> MESHVKYLDELILAIKDLNSGVDSKVQIKKVPTDPSSSQEYAKSLKILNTLIRNLKDQRRNNIMKNDTIFSKTVSALALLLEYNPFLLVMKDSNGNFEIQRLIDDFLNISVLNYDNYHRIWFMRRKLGSWCKACVEFYGKPAKFQLTAHFENTMNLYEQALTEVLLGKTELLKFYDTLKGLYILLYWFTSEYSTFGNSIAFLDSSLGFTKFDFNFQRLIRIVLYVFDSCELAALEYAEIQLKYISLVVDY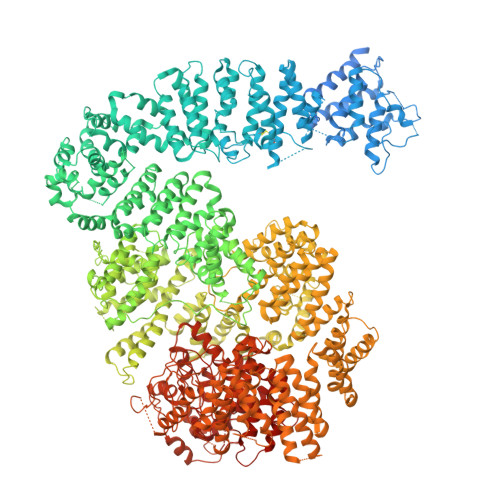VCNRTISTALDAPALVCCEQLKFVLTTMHHFLDNKYGLLDNDPTMAKGILRLYSLCISNDFSKCFVDHFPIDQWADFSQSEHFPFTQLTNKALSIVYFDLKRRSLPVEALKYDNKFNIWVYQSEPDSSLKNVTSPFDDRYKQLEKLRLLVLKKFNKTERGTLLKYRVNQLSPGFFQRAGNDFKLILNEASVSIQTCFKTNNITRLTSWTVILGRLACLESEKFSGTLPNSTKDMDNWYVCHLCDIEKTGNPFVRINPNRPEAAGKSEIFRILHSNFLSHPNIDEFSESLLSGILFSLHRIFSHFQPPKLTDGNGQINKSFKLVQKCFMNSNRYLRLLSTRIIPLFNISDSHNSEDEHTATLIKFLQSQKLPVVKENLVIAWTQLTLTTSNDVFDTLLLKLIDIFNSDDYSLRIMMTLQIKNMAKILKKTPYQLLSPILPVLLRQLGKNLVERKVGFQNLIELLGYSSKTILDIFQRYIIPYAIIQYKSDVLSEIAKIMCDGDTSLINQMKVNLLKKNSRQIFAVALVKHGLFSLDILETLFLNRAPTFDKGYITAYLPDYKTLAEITKLYKNSVTKDASDSENANMILCSLRFLITNFEKDKRHGSKYKNINNWTDDQEQAFQKKLQDNILGIFQVFSSDIHDVEGRTTYYEKLRVINGISFLIIYAPKKSIISALAQISICLQTGLGLKEVRYEAFRCWHLLVRHLNDEELSTVIDSLIAFILQKWSEFNGKLRNIVYSILDTLIKEKSDLILKLKPYTTLALVGKPELGILARDGQFARMVNKIRSTTDLIPIFANNLKSSNKYVINQNLDDIEVYLRRKQTERSIDFTPKKVGQTSDITLVLGALLDTSHKFRNLDKDLCEKCAKCISMIGVLDVTKHEFKRTTYSENEVYDLNDSVQTIKFLIWVINDILVPAFWQSENPSKQLFVALVIQESLKYCGLSSESWDMNHKELYPNEAKLWEKFNSVSKTTIYPLLSSLYLAQSWKEYVPLKYPSNNFKEGYKIWVKRFTLDLLKTGTTENHPLHVFSSLIREDDGSLSNFLLPYISLDIIIKAEKGTPYADILNGIIIEFDSIFTCNLEGMNNLQVDSLRMCYESIFRVFEYCKKWATEFKQNYSKLHGTFIIKDTKTTNMLLRIDEFLRTTPSDLLAQRSLETDSFERSALYLEQCYRQNPHDKNQNGQLLKNLQITYEEIGDIDSLDGVLRTFATGNLVSKIEELQYSENWKLAQDCFNVLGKFSDDPKTTTRMLKSMYDHQLYSQIISNSSFHSSDGKISLSPDVKEWYSIGLEAANLEGNVQTLKNWVEQIESLRNIDDREVLLQYNIAKALIAISNEDPLRTQKYIHNSFRLIGTNFITSSKETTLLKKQNLLMKLHSLYDLSFLSSAKDKFEYKSNTTILDYRMERIGADFVPNHYILSMRKSFDQLKMNEQADADLGKTFFTLAQLARNNARLDIASESLMHCLERRLPQAELEFAEILWKQGENDRALKIVQEIHEKYQENSSVNARDRAAVLLKFTEWLDLSNNSASEQIIKQYQDIFQIDSKWDKPYYSIGLYYSRLLERKKAEGYITNGRFEYRAISYFLLAFEKNTAKVRENLPKVITFWLDIAAASISEAPGNRKEMLSKATEDICSHVEEALQHCPTYIWYFVLTQLLSRLLHSHQSSAQIIMHILLSLAVEYPSHILWYITALVNSNSSKRVLRGKHILEKYRQHSQNPHDLVSSALDLTKALTRVCLQDVKSITSRSGKSLEKDFKFDMNVAPSAMVVPVRKNLDIISPLESNSMRGYQPFRPVVSIIRFGSSYKVFSSLKKPKQLNIIGSDGNIYGIMCKKEDVRQDNQYMQFATTMDFLLSKDIASRKRSLGINIYSVLSLREDCGILEMVPNVVTLRSILSTKYESLKIKYSLKSLHDRWQHTAVDGKLEFYMEQVDKFPPILYQWFLENFPDPINWFNARNTYARSYAVMAMVGHILGLGDRHCENILLDIQTGKVLHVDFDCLFEKGKRLPVPEIVPFRLTPNLLDALGIIGTEGTFKKSSEVTLALMRKNEVALMNVIETIMYDRNMDHSIQKALKVLRNKIRGIDPQDGLVLSVAGQTETLIQEATSEDNLSKMYIGWLPFW>[4x]MSVFSLKIDIADNKFFNGETSPLFSQSQAKLARQFHQKIAGYRPTPLCALDDLANLFGVKKILVKDESKRFGLNAFKMLGGAYAIAQLLCEKYHLDIETLSFEHLKNAIGEKMTFATTTDGNHGRGVAWAAQQLGQNAVIYMPKGSAQERVDAI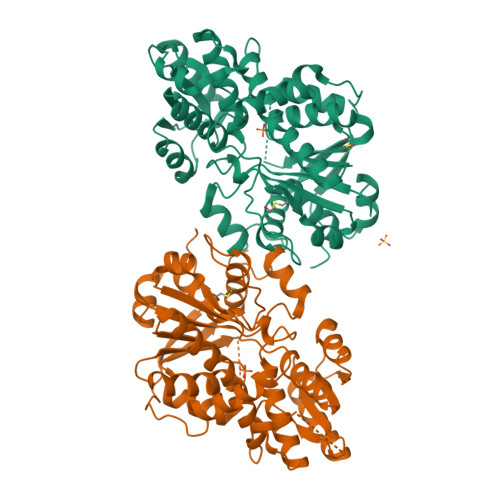LNLGAECIVTDMNYDDTVRLTMQHAQQHGWEVVQDTAWEGYTKIPTWIMQGYATLADEAVEQMREMGVTPTHVLLQAGVGAMAGGVLGYLVDVYSPQNLHSIIVEPDKADCIYRSGVKGDIVNVGGDMATIMAGLACGEPNPLGWEILRNCATQFISCQDSVAALGMRVLGNPYGNDPRIISGESGAVGLGVLAAVHYHPQRQSLMEKLALNKDAVVLVISTEGDTDVKHYREVVWEGKHAVAP ALPHA-AMINOBUTYRIC 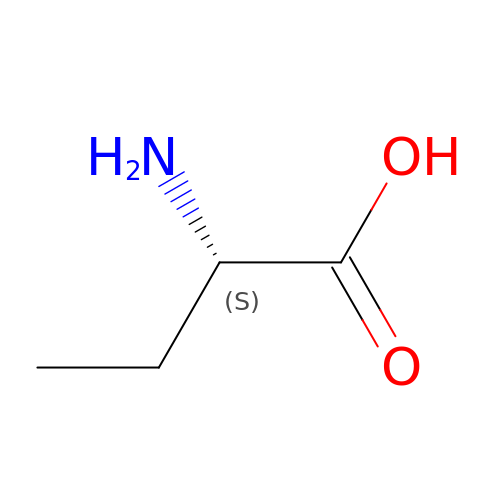ACID | C4 H9 N O2 | QWCKQJZIFLGMSD-VKHMYHEASA-N>MSRLVVVSNRIAPPDEHAASAGGLAVGILGALKAAGGLWFGWSGETGNEDQPLKKVKKGNITWASFNLSEQDLDEYYNQFSNAVLWPAFHYRLDLVQFQRPAWDGYLRVNALLADKLLPLLQDDDIIWIHDYHLLPFAHELRKRGVNNRIGFFLHIPFPTPEIFNALPTYDTLLEQLCDYDLLGFQTENDRLAFLDCLSNLTRVTTRSAKSHTAWGKAFRTEVYPIGIEPKEIAKQAAGPLPPKLAQLKAELKNVQNIFSVERLDYSKGLPERFLAYEALLEKYPQHHGKIRYTQIAPTSRGDVQAYQDIRHQLENEAGRINGKYGQLGWTPLYYLNQHFDRKLLMKIFRYSDVGLVTPLRDGMNLVAKEYVAAQDPANPGVLVLSQFAGAANELTSALIVNPYDRDEVAAALDRALTMSLAERISRHAEMLDVIVKNDINHWQECFISDLKQIVP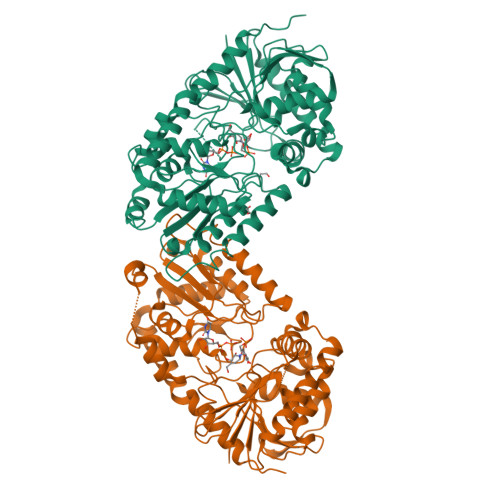RSAESQQRDKVATFPKLA[4x]> MSLTFNENGVQTNTFSELRALLEAGYREIYGTDIVTDQESPDGQRINLETLLRFDIESAFSWLYSNLDPDLNTGDMQQIIGKLSGLVLLPASRSQWDVTINMSRAKTLPAGYTITDENNQNWFLDSDVDVLIGDNEVTFLSSLWGSISGISGSSFTQATPEIGVVSISASADAIQGREEETPEQFRLRRQRSTENPAQSTIGSIYAKLAQINGVTDLQVYDNSSDTPDQITGSSNPDILNGSEPVTIGAHTMWVVIEGGSLDDIGEVVAKHRLGNTKGSVQVSYIDTLTKPNGDDFQIVNLHNIDRPVLGDLYVRLTATQKVSGSPIDTDAIKNKLSLVDFEIGQYVDADALYQQSLITNSNYNVTDLEVSLNGID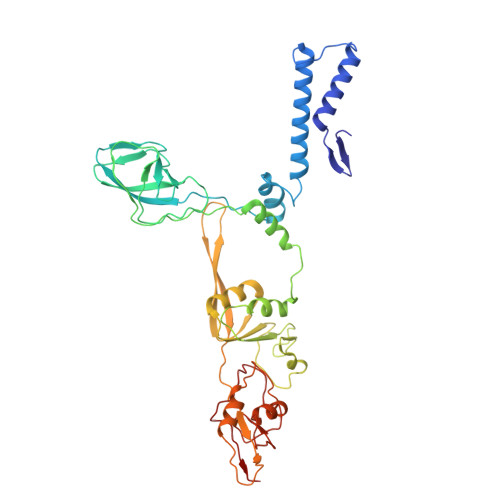WTDGRVFSGYDGKLSISTSNVTITTVPV Lectins are carbohydrate binding proteins unrelated to immunoglobulins that display no enzymatic activity towards the recognized sugars. Lectins purified from seeds of the Diocleinae subtribe exhibit a high degree of sequence identity notwithstanding that they show very distinct biological activities. In the present study, we used mass spectrometry to determine the amino acid sequence of a lectin from Canavalia boliviana seeds and solved its crystal structure in complex with Xman and the dimannosides Man(α1-3)Man(α1-O)Me and Man(α1-4)Man(α1-O)Me. Furthermore, we characterized the anti-inflammatory properties of Cbol, adding more data to the repertoire of wide biological activities displayed by this group of lectins, despite their highly identical sequence.

The carbohydrate electron densities of M13M and M14M and Xman complexes are well defined in all subunits. In Cbol:Xman, however, extensive interactions are observed in the binding region. The O1-linked mannose of both dimannosides, M13M and M14M, as well as Xman, are bound to the monosaccharide binding site in an almost identical way to that observed for ConA, CGL and ConM. Other than in the carbohydrate-binding region, the complexes do not present any significant structural differences when compared to the unbound protein.

> ADTIVAVELDTYPNTDIGDPSYPHIGIDIKSVRSKKTAKWNMQNGKVGTAHIIYNSVGKRLSAVVSYPNGDSATVSYDVDLDNVLPEWVRVGLSATTGLYKETNTILSWSFTSKLKSNSTHETNALHFMFNQFSKDQKDLILQGDATTGRDGNLELTRVSSNGSPQGSSVGRALFYAPVHIWESSAVVASFDATFTFLIKSSDSHPADGIAFFISNIDSSIPSGSTGRLLGLFPDAN(3R)-N-(2-formylindolizin-3-yl)-4-[(phenylacetyl)oxy]-3-sulfino-D-valine | C22 H22 N2 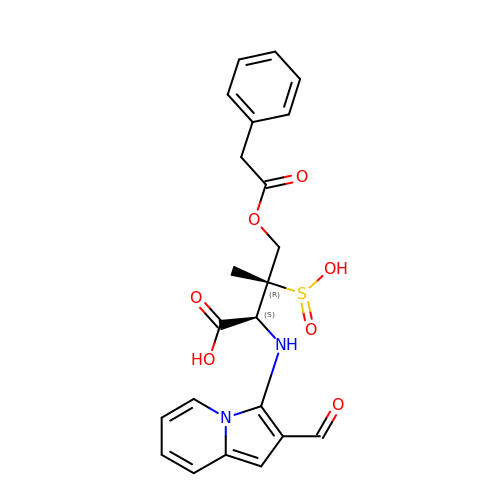O7 S | WQTYZCOJEVFYJF-UGKGYDQZSA-N>MNNLYRDLAPVTEAAWAEIELEAARTFKRHIAGRRVVDVSDPGGPVTAAVSTGRLIDVKAPTNGVIAHLRASKPLVRLRVPFTLSRNEIDDVERGSKDSDWEPVKEAAKKLAFVEDRTIFEGYSAASIEGIRSASSNPALTLPEDPREIPDVISQALSELRLAGVDGPYSVLLSADVYTKVSETSDHGYPIREHLNRLVDGDIIWAPAIDGAFVLTTRGGDFDLQLGTDVAIGYASHDTDTVRLYLQETLTFLCYTAEASVALSHKLAAAALEHHHHHH[20x];>[9x]MAVPAVSPQPILAPLTPAAIFLVATIGADGEATVHDALSKISGLVRAIGFRDPTKHLSVVVSIGSDAWDRLFAGPRPTELHPFVELTGPRHTAPATPGDLLFHIRAETMDVCFELAGRILKSMGDAVTVVDEVHGFRFFDNRDLLGFVDGTENPSGPIAIKATTIGDEDRNFAGSCYVHVQKYVHDMASWESLSVTEQERVIGRTKLDDIELDDNAKPANSHVALNVITDDDGTERKIVRHNMPFGEVGKGEYGTYFIGYSRTPTVTEQMLRNMFLGDPAGNTDRVLDFSTAVTGGLFFSPTIDFLDHPPPLPQAATPTLAAGSLSIGSLKGSPR

Dye-decolorizing peroxidase (DyP), an enzyme involved in Mtb’s oxidative stress response, is encapsulated in a nanocompartment, encapsulin (Enc), and is important for Mtb’s survival in macrophages. Enc nanocompartments self-assemble to form a protein shell with icosahedral symmetry. The Enc protein is a homolog of a single subunit viral capsid protein and adopts a HK97 (bacteriophage Hong Kong 97)-like fold. DyP is a heme-containing enzyme that oxidizes and degrades a wide range of synthetic dyes and, importantly, reduces hydrogen peroxide (H2O2) to water. It has been shown that Mtb-DyP is a hexamer, where the C-terminus of Mtb-DyP contains the TP sequence that targets Mtb-DyP to the interior of the Mtb-Enc 60-mer shell.

The crystal structure of the Mtb-Enc•DyP complex was solved by MR to 3.15 Å resolution and refined to a final Rwork/Rfree of 20.2/23.3. Application of crystallographic symmetry generated an intact 60-subunit capsule with T1 icosahedral symmetry. While the compact domain of Mtb-DyP (residues 1-314 based on the AlphaFold Mtb-DyP predicted structure) lacks a corresponding electron density in the interior of the Mtb-Enc shell and cannot be modeled, the electron density for Mtb-DyP-TP was observed. In the ASU, nine DyP-TPs were modeled. These peptides were bound to the interior of subunits D, G, H, I, P, Q, R, S, and T, and are referred to as d, g, h, i, p, q, r, s, and t, respectively. In addition to the Mtb-DyP-TPs, the Mtb-Enc•DyP structure displayed excess electron density that we modeled with molecules from the purification and crystallization process: glycerol, nickel (Ni2+) ions, and PEG molecules. Notably, the crystal structure of Mtb-Enc•DyP described here has the smallest mycobacterial five-fold pore described to date at 3.6 A. In the crystal structure, the Cα of His187 is translated ~5–6 Å upwards, resulting in the orientation of its carbonyl oxygen directly into the pore, and Tyr189 is angled ~45–50° along the pore and translated such that the hydroxyl group is ~6–7 Å away from its cryo-EM position. Further, when investigating areas where small molecules from the purification buffer or crystallographic condition colocalize, we noted intriguing small pores formed at the interface of neighboring subunits along the five-fold symmetry axis, which will be referred to as five-fold minor pores, while the pore formed at the five-fold symmetry axis will be referred to as the five-fold major pore. The resulting pore has, on average, a bottleneck diameter of 3.4 ± 0.8 Å, with −1.8 ± 0.4 hydropathy and 26.6 ± 4.1 polarity.> GMKQSKKIIITCAVTGSIHTPTMSPYLPITPEEIVKEGVAAAEAGAAMLHLHARDPLNGRPSQDPDLFMRFLPQLKERTDAILNITTGG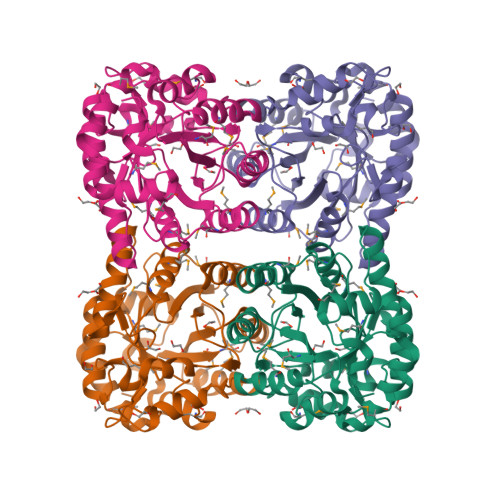GLGMSLDERLAPARAARPEVASMNMGSLNFNISQAAAKFDTFKFDWERPYLAGTRDFILSNTFSQIERGMTELGASGTRFEFECYDVGHLYNLAHFVDRKLVEPPFFLQCVFGILGGIGADPENLLHMRTIADRLFGQDYYLSVLAAGRHQMPFVTMSAILGGNVRVGLEDSLYSGKGQLATSNAEQVRKIRRIIEELSLDIATPDEARAMLKTKGANETSF> GSHMTRLAPVVVDVPDDVLVLRVIGPLFFAAAEGLFTDLESRLEGKRIVILKWDAVPVLDAGGLDAFQRFVKRLPEGCE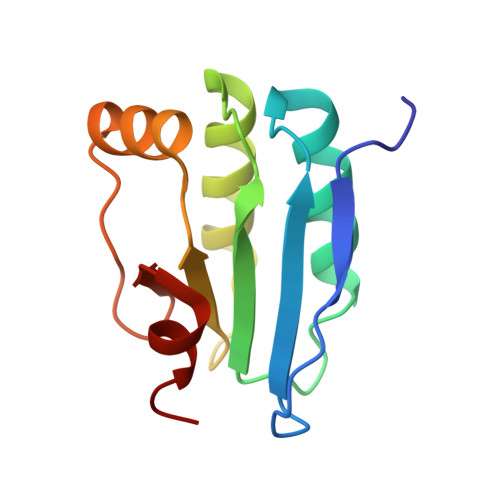LRVCNVEFQPLRTMARAGIQPIPGRLAFFPNRRAAMADL>[6x]MAAPARDPPGYRYAAAILPTGSILSTIEVASHRRLFDFFAAVRSDENSLYDVEFDALLGSYCNTLSLVRFLELGLSVACVCTKFPELAYMNEGRVQFEVHQPLIARDGPHPVEQPVHNYMTKVIDRRALNAAFSLATEAIALLTGEALDGTGISLHRQLRAIQQLARNVQAVLGAFERGTADQMLHVLLEKAPPLALLLPMQRYLDNGRLATRVARATLVAELKRSFCDTSFFLGKAGHRREAIEAWLVDLTTATQPSVAVPRLTHADTRGRPVDGVLVTTAAIKQRLLQSFLKVEDTEADVPVTYGEMVLNGANLVTALVMGKAVRSLDDVGRHLLDMQEEQLEANRETLDELESAPQTTRVRADLVAIGDRLVFLEALERRIYAATNVPYPLVGAMDLTFVLPLGLFNPAMERFAAHAGDLVPAPGHPEPRAFPPRQLFFWGKDHQVLRLSMENAVGTVCHPSLMNIDAAVGGVNHDPVEAANPYGAYVAAPAGPGADMQQRFLNAWRQRLAHGRVRWVAECQMTAEQFMQPDNANLALELHPAFDFFAGVADVELPGGEVPPAGPGAIQATWRVVNGNLPLALCPVAFRDARGLELGVGRHAMAPATIAAVRGAFEDRSYPAVFYLLQAAIHGNEHVFCALARLVTQCITSYWNNTRCAAFVNDYSLVSYIVTYLGGDLPEECMAVYRDLVAHVEALAQLVDDFTLPGPELGGQAQAELNHLMRDPALLPPLVWDCDGLMRHAALDRHRDCRIDAGGHEPVYAAACNVATADFNRNDGRLLHNTQARAADAADDRPHRPADWTVHHKIYYYVLVPAFSRGRCCTAGVRFDRVYATLQNMVVPEIAPGEECPSDPVTDPAHPLHPANLVANTVKRMFHNGRVVVDGPAMLTLQVLAHNMAERTTALLCSAAPDAGANTASTANMRIFDGALHAGVLLMAPQHLDHTIQNGEYFYVLPVHALFAGADHVANAPNFPPALRDLARDVPLVPPALGANYFSSIRQPVVQHARESAAGENALTYALMAGYFKMSPVALYHQLKTGLHPGFGFTVVRQDRFVTENVLFSERASEAYFLGQLQVARHETGGGVNFTLTQPRGNVDLGVGYTAVAATGTVRNPVTDMGNLPQNFYLGRGAPPLLDNAAAVYLRNAVVAGNRLGPAQPLPVFGCAQVPRRAGMDHGQDAVCEFIATPVATDINYFRRPCNPRGRAAGGVYAGDKEGDVIALMYDHGQSDPARPFAATANPWASQRFSYGDLLYNGAYHLNGASPVLSPCFKFFTAADITAKHRCLERLIVETGSAVSTATAASDVQFKRPPGCRELVEDPCGLFQEAYPITCASDPALLRSARDGEAHARETHFTQYLIYDASPLKGLSL;> MNAHFANEVQYDLTRDPSSPASLIHVIISSECLAAAGVPLSALMRGRPDGGAAANFRVETQTRAHATGDCTPWRSAFAAYVPADAVGALIAPVVPAHPDLLPRVPSAGGLFVSLPVACDAQGVYDPYTVAALRLAWGPWATCARVLLFSYDELVPPNTRYAADGARLMRLCRHFCRYVARLGAAAPAAATEAAAHLSMGLGESGTPTPQASSVSGGAGPAVVGTPDPPISPEEQLTAPGGDTATAEDVSITQENEEILALVQRAVQDVTRRHPVRARPKHAASGVASGLRQGALVHQAVSGGALGASDAEAVLAGLEPPGGGRFASRGGPRAAGEDVLNDVLTLVPGTAKPRSLVEWLDRGWEALAGGDRPDWLWSRRSISVVLRHHYGTKQRFVVVSYENSVAWGGRRARPPRLSSELATALTEACAAERVVRPHQLSPAAQTALLRRFPALEGPLRHPRPVLQPFDIAAEVAFVARIQIACLRALGHSIRAALQGGPRIFQRLRYDFGPHQSEWLGEVTRRFPVLLENLMRALEGTAPDAFFHTAYALAVLAHLGGQGGRGRRRRLVPLSDDIPARFADSDAHYAFDYYSTSGDTLRLTNRPIAVVIDGDVNGREQSKCRFMEGSPSTAPHRVCEQYLPGESYAYLCLGFNRRLCGLVVFPGGFAFTINTAAYLSLADPVARAVGLRFCRGAATGPGLVR;>MDPYYPFDALDVWEHRRFIVADSRSFITPEFPRDFYMSPVFNIPRETAAERAAVLQAQRTAAAAALENAALQAAELPVDIERRIRPIEQQVHHIADALEALETAATAAEEADAARDAEARGEGAADGAAPSPTAGPAAAEMEVQIVRNDPPLRYDTNLPVDLLHMVYAGRGAAGSSGVVFGTWYRTIQERTIADFPLTTRSADFRDGRMSKTFMTALVLSLQSCGRLYVGQRHYSAFECAVLCLYLLYRTTHESSPDRDRAPVAFGDLLARLPRYLARLAAVIGDESGRPQYRYRDDKLPKAQFAAAGGRYEHGALATHVVIATLVRHGVLPAAPGDVPRDTSTRVNPDDVAHRDDVNRAAAAFLARGHNLFLWEDQTLLRATANTITALAVLRRLLANGNVYADRLDNRLQLGMLIPGAVPAEAIARGASGLDSGAIKSGDNNLEALCVNYVLPLYQADPTVELTQLFPGLAALCLDAQAGRPLASTRRVVDMSSGARQAALVRLTALELINRTRTNTTPVGEIINAHDALGIQYEQGLGLLAQQARIGLASNAKRFATFNVGSDYDLLYFLCLGFIPQYLSVA[2x];>MAAPQFHRPSTITADNVRALGMRGLVLATNNAQFIMDNSYPHPHGTQGAVREFLRGQAAALTDLGVTHANNTFAPQPMFAGDAAAEWLRPSFGLKRTYSPFVVRDPKTPSTP[6x];>MIPAALPHPTMKRQGDRDIVVTGVRNQFATDLEPGGSVSCMRSSLSFLSLLFDVGPRDVLSAEAIEGCLVEGGEWTRAAAGSGPPRMCSIIELPNFLEYPAARGGLRCVFSRVYGEVGFFGEPTAGLLETQCPAHTFFAGPWAMRPLSYTLLTIGPLGMGLYRDGDTAYLFDPHGLPAGTPAFIAKVRAGDVYPYLTYYAHDRPKVRWAGAMVFFVPSGPGAVAPADLTAAALHLYGASETYLQDEPFVERRVAITHPLRGEIGGLGALFVGVVPRGDGEGSGPVVPALPAPTHVQTPGADRPPEAPRGASGPPDTPQAGHPNRPPDDVWAAALEGTPPAKPSAPDAAASGPPHAAPPPQTPAGDAAEEAEDLRVLEVGAVPVGRHRARYSTGLPKRRRPTWTPPSSVEDLTSGERPAPKAPPAKAKKKSAPKKKAPVAAEVPASSPTPIAATVPPAPDTPPQSGQGGGDDGPASPSSPSVLETLGARRPPEPPGADLAQLFEVHPNVAATAVRLAARDAALAREVAACSQLTINALRSPYPAHPGLLELCVIFFFERVLAFLIENGARTHTQAGVAGPAAALLDFTLRMLPRKTAVGDFLASTRMSLADVAAHRPLIQHVLDENSQIGRLALAKLVLVARDVIRETDAFYGDLADLDLQLRAAPPANLYARLGEWLLERSRAHPNTLFAPATPTHPEPLLHRIQALAQFARGEEMRVEAEAREMREALDALARGVDSVSQRAGPLTVMPVPAAPGAGGRAPCPPALGPEAIQARLEDVRIQARRAIESAVKEYFHRGAVYSAKALQASDSHDCRFHVASAAVVPMVQLLESLPAFDQHTRDVAQRAALPPPPPLATSPQAILLRDLLQRGQPLDAPEDLAAWLSVLTDAATQGLIERKPLEELARSIHGINDQQARRSSGLAELQRFDALDAALAQQLDSDAAFVPATGPAPYVDGGGLSPEATRMAEDALRQARAMEAAKMTAELAPEARSRLRERAHALEAMLNDARERAKVAHDAREKFLHKLQGVLRPLPDFVGLKACPAVLATLRASLPAGWTDLADAVRGPPPEVTAALRADLWGLLGQYREALEHPTPDTATALAGLHPAFVVVLKTLFADAPETPVLVQFFSDHAPTIAKAVSNAINAGSAAVATASPAATVDAAVRAHGALADAVSALGAAARDPASPLSFLAVLADSAAGYVKATRLALEARGAIDELTTLGSAAADLVVQARRACAQPEGDHAALIDAAARATTAARESLAGHEAGFGGLLHAEGTAGDHSPSGRALQELGKVIGATRRRADELEAAVADLTAKMAAQRARGSSERWAAGVEAALDRVENRAEFDVVELRRLQALAGTHGYNPRDFRKRAEQALAANAEAVTLALDTAFAFNPYTPENQRHPMLPPLAAIHRLGWSAAFHAAAETYADMFRVDAEPLARLLRIAEGLLEMAQAGDGFIDYHEAVGRLADDMTSVPGLRRYVPFFQHGYADYVELRDRLDAIRADVHRALGGVPLDLAAAAEQISAARNDPEATAELVRTGVTLPCPSEDALVACAAALERVDQSPVKNTAYAEYVAFVTRQDTAETKDAVVRAKQQRAEATERVMAGLREALAARERRAQIEAEGLANLKTMLKVVAVPATVAKTLDQARSVAEIADQVEVLLDQTEKTRELDVPAVIWLEHAQRTFETHPLSAARGDGPGPLARHAGRLGALFDTRRRVDALRRSLEEAEAEWDEVWGRFGRVRGGAWKSPEGFRAMHEQLRALQDTTNTVSGLRAQPAYERLSARYQGVLGAKGAERAEAVEELGARVTKHTALCARLRDEVVRRVPWEMNFDALGGLLAEFDAAAADLAPWAVEEFRGARELIQYRMGLYSAYARAGGQTGAGAESAPAPLLVDLRALDARARASSSPEGHEVDPQLLRRRGEAYLRAGGDPGPLVLREAVSALDLPFATSFLAPDGTPLQYALCFPAVTDKLGALLMRPEAACVRPPLPTDVLESAPTVTAMYVLTVVNRLQLALSDAQAANFQLFGRFVRHRQATWGASMDAAAELYVALVATTLTREFGCRWAQLGWASGAAAPRPPPGPRGSQRHCVAFNENDVLVALVAGVPEHIYNFWRLDLVRQHEYMHLTLERAFEDAAESMLFVQRLTPHPDARIRVLPTFLDGGPPTRGLLFGTRLADWRRGKLSETDPLAPWRSALELGTQRRDVPALGKLSPAQALAAVSVLGRMCLPSAALAALWTCMFPDDYTEYDSFDALLAARLESGQTLGPAGGREASLPEAPHALYRPTGQHVAVLAAATHRTPAARVTAMDLVLAAVLLGAPVVVALRNTTAFSRESELELCLTLFDSRPGGPDAALRDVVSSDIETWAVGLLHTDLNPIENACLAAQLPRLSALIAERPLADGPPCLVLVDISMTPVAVLWEAPEPPGPPDVRFVGSEATEELPFVATAGDVLAASAADADPFFARAILGRPFDASLLTGELFPGHPVYQRPLADEAGPSAPTAARDPRDLAGGDGGSGPEDPAAPPARQADPGVLAPTLLTDATTGEPVPPRMWAWIHGLEELASDDAGGPTPNPAPALLPPPATDQSVPTSQYAPRPIGPAATARETRPSVPPQQNTGRVPVAPRDDPRPSPPTPSPPADAALPPPAFSGSAAAFSAAVPRVRRSRRTRAKSRAPRASAPPEGWRPPALPAPVAPVAASARPPDQPPTPESAPPAWVSALPLPPGPASARGAFPAPTLAPIPPPPAEGAVVPGGDRRRGRRQTTAGPSPTPPRGPAAGPPRRLTRPAVASLSASLNSLPSPRDPADHAAAVSAAAAAVPPSPGLAPPTSAVQTSPPPLAPGPVAPSEPLCGWVVPGGPVARRPPPQSPATKPAARTRIRARSVPQPPLPQPPLPQPPLPQPPLPQPPLPQPPLPQPPLPQPPLPQPPLPQPPLPQPPLPPVTRTLTPQSRDSVPTPESPTHTNTHLPVSAVTSWASSLALHVDSAPPPASLLQTLHISSDDEHSDADSLRFSDSDDTEALDPLPPEPHLPPADEPPGPLAADHLQSPHSQFGPLPVQANAVLSRRYVRRTGRSALAVLIRACRRIQQQLQRTRRALFQRSNAVLTSLHHVRMLLG[2x];>[2x]MITDCFEADIAIPSGISRPDAAALQRCEGRVVFLPTIRRQLALADVAHESFVSGGVSPDTLGLLLAYRRRFPAVITRVLPTRIVACPVDLGLTHAGTVNLRNTSPVDLCNGDPVSLVPPVFEGQATDVRLESLDLTLRFPVPLPTPLAREIVARLVARGIRDLNPDPRTPGELPDLNVLYYNGARLSLVADVQQLASVNTELRSLVLNMVYSITEGTTLILTLIPRLLALSAQDGYVNALLQMQSVTREAAQLIHPEAPMLMQDGERRLPLYEALVAWLAHAGQLGDILALAPAVRVCTFDGAAVVQSGDMAPVIRYP;> MKTKPLPTAPMAWAESAVETTTSPRELAGHAPLRRVLRPPIARRDGPVLLGDRAPRRTASTMWLLGIDPAESSPGTRATRDDTEQAVDKILRGARRAGGLTVPGAPRYHLTRQVTLTDLCQPNAERAGALLLALRHPTDLPHLARHRAPPGRQTERLAEAWGQLLEASALGSGRAESGCARAGLVSFNFLVAACAAAYDARDAAEAVRAHITTNYGGTRAGARLDRFSECLRAMVHTHVFPHEVMRFFGGLVSWVTQDELASVTAVCSGPQEATHTGHPGRPCSAVTIPACAFVDLDAELCLGGPGAAFLYLVFTYRQCRDQELCCVYVVKSQLPPRGLEAALERLFGRLRITNTIHGAEDMTPPPPNRNVDFPLAVLAASSQSPRCSASQVTNPQFVDRLYRWQPDLRGRPTARTCTYAAFAELGVMPDDSPRCLHRTERFGAVGVPVVILEGVVWRPGGWRACA

Here we show asymmetric reconstructions of herpes simplex virus 2 (HSV-2) B- (containing scaffold proteins inside, putative capsid assembly intermediate), C- (DNA-filled capsid, derived from the enveloped virion by using detergent treatment to remove viral membrane proteins and outer tegument proteins) and virion-capsids (enveloped intact virion) at 8.1, 9.0 and 10.2 Å respectively. The asymmetric reconstructions reveal a unique portal vertex in the context of the icosahedral capsid, including 1 portal, 11 pentons, 3 types of hexons (P, peripentonal; E, edge; C, center) with the hexameric rings formed by VP26s, 320 triplexes (Ta-Tf) and 12 pentagram-shaped capsid vertex specific component (CVSC) densities (composed of a UL17 monomer, a UL25 dimer and a UL36 dimer, presence in C- and virion-capsids). Radially colored representations of the three reconstructions reveal the dodecameric portal situated beneath one of the pentameric vertices; but, the density surrounding the portal displays a five-fold symmetrical assembly, highlighting the symmetry-mismatch structural features. The portal vertex of the capsid is a hub for protein-protein interactions that are important for capsid assembly and genome packaging.

When five-fold symmetry was imposed, the resolution of local reconstructions for the portal vertex in B-, C- and virion-capsids was improved to 4.05, 4.50 and 5.36 Å, respectively, albeit that the portal was five-fold averaged. The resulting density maps clearly reveal the polypeptide backbone, many bulky side chains, and atomic models of the portal vertex associated P-hexon (PVP-Hex), Ta and PVAT (not in B-capsid) from three capsids were built. Despite distinct organizations of the CVSC at the portal and penton vertices, the packaged dsDNA is visible in the C- and virion-capsids. In contrast to B-capsid, small tail-like density, previously named Portal Vertex Associated Tegument (PVAT), extends outwards from the portal vertex in the C- and virion-capsids, suggesting a possible role in genome retention and release. A comparison of asymmetric reconstructions of the portal vertex of the three capsids reveals notable differences in the position and morphology of the portal and PVAT. Distinct from the virion-capsid, a bulk of obvious densities presumably emanating from dsDNA beneath the portal is observed, however some exterior densities, corresponding to five copies of coiled coils and five copies of the UL25 C domain, become disordered or lost in the C-capsid, consistent with previous observations of the CVSC of HSV-2 C-capsid. These might result from the lack of protection offered by tegument proteins/envelope, indicative of the vulnerability of the role in the retention of viral genome of isolated C-capsids in vitro, reflecting purified C-capsids are metastable and tend to release their genome.>[2x]VKSKAKKTVDKHSDEYKIRRERNNIA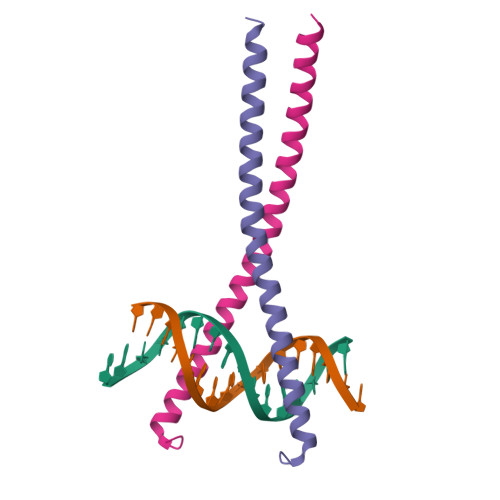ARKSRDKAKMRNLETQHKVLELTAENERLQKKVEQLSRELSTLRNLFKQLPE(4-{[(1R,2R)-2-(carboxymethyl)cyclopentyl]methyl}phenyl)acetic 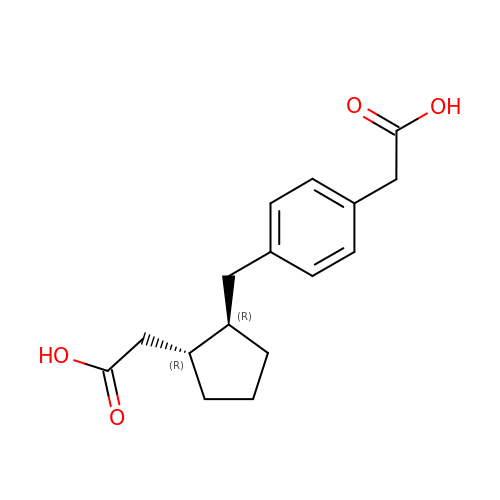acid | C16 H20 O4 | QKXFMUHRVZWRPO-ZIAGYGMSSA-N> MGRQIPPDPVFGDVLVAKLINRVMWDGKKTIAQKIVYGAFDIIREKTKKDPLEVFRQAVENVKPVLEVRPRRVGGATYQVPIEVQEPRRTSLALRWIVEAARAKKGRPMKEKL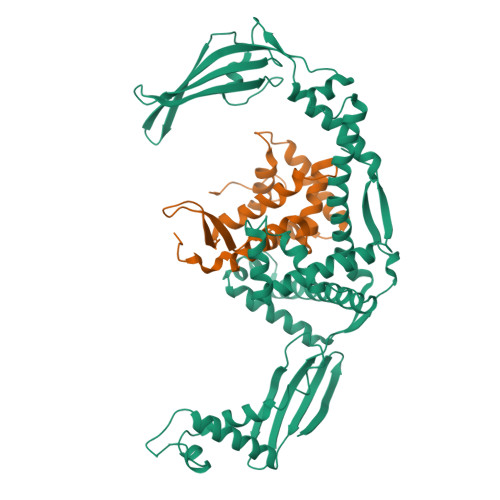AEEIIAAYNNTGTAIKKKEDTHRMAEANRAFAHYRW;> MEVKELERDKNRVVLEYVFGAEEIAQAEDKAVRYLNQRVEIPGFRKGRIPKNVLKMKLGEEFQEYTLDFLMDLIPDTLKDRKLILSPIVTERELKDVTARVVVEVHEEPEVRIGDISKIEVEKVDEEKVLEKYVERRIEDLRESHALLEPKEGPAEAGDLVRVNMEVYNEEGKKLTSREYEYVISEDEDRPFVKDLVGKKKGDVVEIEREYEGKKYTYKLEVEEVYKRTLPEIGDELAKSVNNEFETLEQLKESLKKEGKEIYDVEMKESMREQLLEKLPEIVEIEISDRTLEILVNEAINRLKREGRYEQIVSSYESEEKFREELKERILDDIKRDRVIEVLAQEKGISVNDEELEKEAEELAPFWGISPDRAKSLVKARQDLREELRWAILKRKVLDLLLQEVKVKVVEPKGEGDDSEGKEDNLEHHHHHH> CAAAGAAAAG;> CTTTTCTTT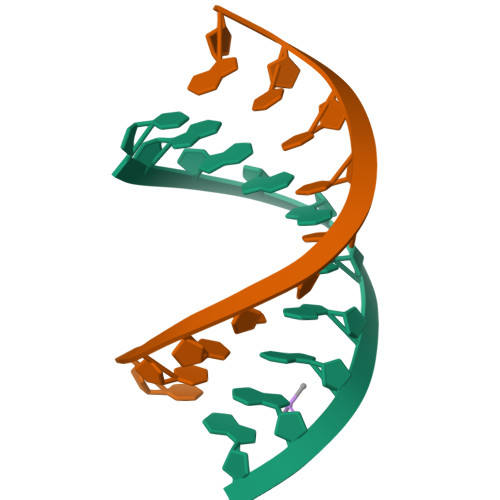G> MHHHHHHSSGRENLYFQGSKPRILLMGLRRSGKSSIQKVVFHKMSPNETLFLESTNKIYKDDISNSSFVNFQIWDFPGQMDFFDPTFDYEMIFRGTGALIYVIDAQDDYMEALTRLHITVSKAYKVNPDMNFEV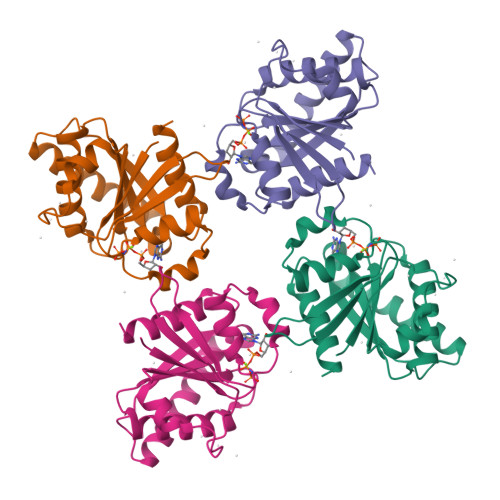FIHKVDGLSDDHKIETQRDIHQRANDDLADAGLEKLHLSFYLTSIYDHSIFEAFSKVVQKLI ethyl 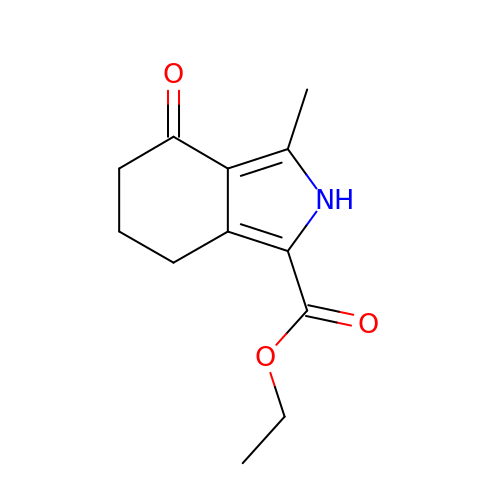3-methyl-4-oxo-4,5,6,7-tetrahydro-2H-isoindole-1-carboxylate | C12 H15 N O3 | QMQMLKBVJSOVCI-UHFFFAOYSA-N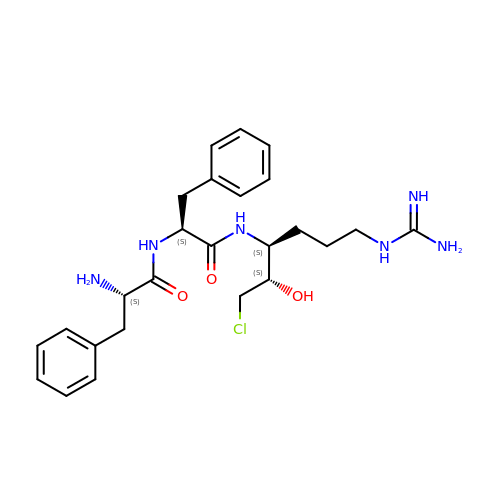L-phenylalanyl-N-[(2S,3S)-6-carbamimidamido-1-chloro-2-hydroxyhexan-3-yl]-L-phenylalaninamide | C25 H35 Cl N6 O3 | ZKHBINZTIMXMQW-MYGLTJDJSA-N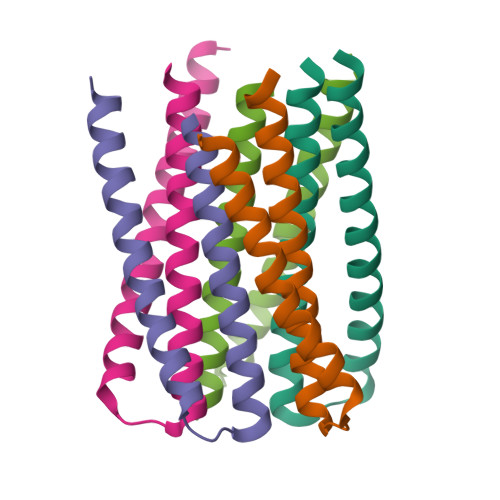>GSHMTRRKQEMKRLKYEMEKIREETEEVKKEIEESKKRPQSESAKNLILIMQLLINQIRLLALQIRMLALQLQE[10x]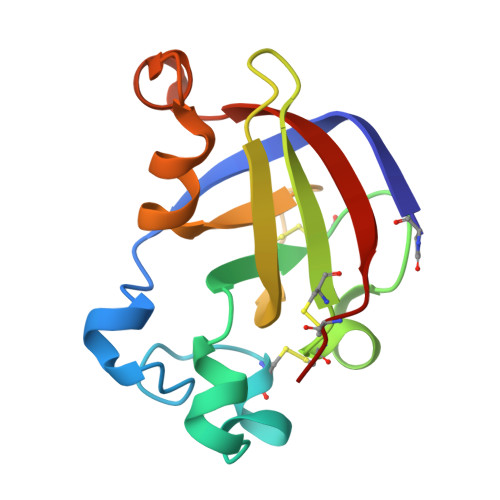> QSASNVRATYHFYNAQQNGWDLRKVSAYCATWDADKPYSWRSKYGWTAFCGPVGPHGRAACGKCLRVTNTKTRAETTVRIVDQCSNGGLDLDWSVFKKLDTDGSGYLRGHLIVNYQFVNCGN> MSYYHHHHHHLESTSLYKKAGSAAAPFTMANENSNKEIVKEVLPLIRVYKDGTVERLLSSPNVAASPEDPETGVSSKDIVIAHNPYVSARIFLPNINKSHNKLPIFVYFHGGAFCVESAFSFFVHRYLNILASQANIIAVSVDFRLLPHHPLPAAYEDGWTTLQWIASHANNTATNPEPWLLNHADFNKLYVGGETSGANLAHNLLLRAGNGNQSLP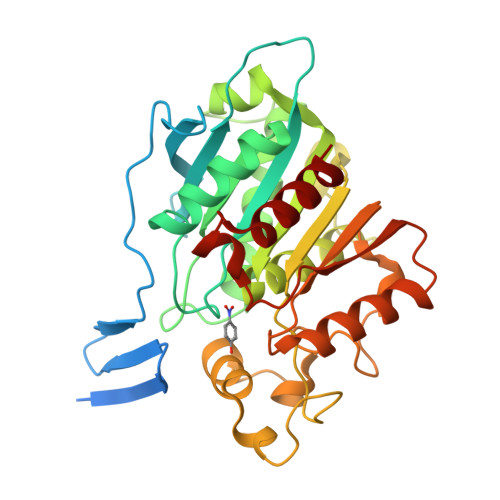GDLKILGGLLCCPFFWGSKPIGSEPVDEHEQSLAMKVWNLACPDAPGGIDNPWINPCVAGAPSLATLGCSKLLVTITGRDEFRDRDILYHDTVKKSGWEGQLELFDAGDEEHAFQLFKPETDTAKAMIKRLASFLV> MKPPQFTWAQWFETQHINMTSQQCTNAMQVINNYQRRCKNQNTFLLTTFANVVNVCGNPNMTCPSNKTRKNCHHSGSQVPLIHCNLTTPSP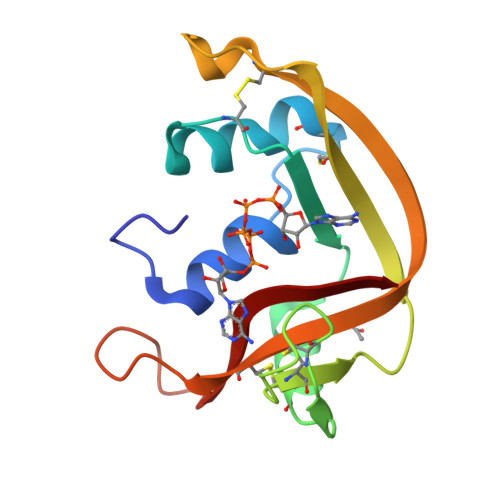QNISNCRYAQTPANMFYIVACDNRDQRRDPPQYPVVPVHLDRII>[2x]MKPHNSEKYFVKNGQPHFLISGEVHYFRINPKLWRNHLQLLKQTGADTVSTYIPWDWHEIEEDDFDFEGKTHPARNLIRFIKLCKEENLDLIVKPGPYILAEYENQGLPSWLLKKLSKNAFALDENGNVISPDLVSYLSDEFLEYTFKWYDKVMPIISKHQKEHYGPITMMQLCNEIGVFQWLSGKSDYNPKVINLYKEFIIQRYKTIEKLNSVYSTNYNSFDDLKAPSGKIKLRSDYCAYFDFHLFFREYYNKYISILKNKIRSFGINIKLTHNIPGWIYGNASELPMLISTYSEIMKNHPDIIFGLDHIPEFVSFRNAHSDLACNKILEAMQPEAPVWAAQFQAGTREHHVKAYAKDLETFYIASLAHGIKGFNYYMFSQGINPEGKGFYGKTFYFQTALDAASNKLALYDSIKKVNRFIRKEQKDLLRTNVNSEICVGFYKPYFFTELISSQLLKEKKLNVEELGLYIDPRFLREEILFNGLLRGLQTLNYNYDVVDLENCDLKSLTAYKQLWITSAEFMDAETQNLLSEFVLNGGNLILYPAVPTLDNYLNRCEILKNNFGIEFITKDSSHKVSAFGIEDVFTAFSKKQIYNDTNSKPIAFTQENEICGIRKKIGKGELTILGFAFGYTSDEHLELIDKLVKLNKIKRELFVSDKDIQFVVRENNKSRYIFFLNYHNERKTFNYRKSSELKKKKSEEISIAPFSYKVIKENKLEHHHHHH

The IALB_1185 protein, which is encoded in the gene cluster for endo-β-1,2-glucanase homologs in the genome of Ignavibacterium album, is a glycoside hydrolase family (GH) 35 protein. Here, we showed using recombinant IALB_1185 that this protein has glycosyltransferase activity toward β-1,2-glucooligosaccharides, and that the kinetic parameters for β-1,2-glucooligosaccharides are not within the ranges for general GH enzymes. Kinetic analysis further revealed that the enzyme has wide aglycone specificity regardless of the anomer, and that the β-1,2-linked glucose dimer sophorose is an appropriate donor. We propose that IALB_1185 be redefined β-1,2-glucooligosaccharide:d-glucoside β-d-glucosyltransferase as a systematic name and β-1,2-glucosyltransferase as an accepted name.

Thus, crystals of the E343Q mutant (the mutant of the nucleophile) were soaked in a solution containing Sop4. Clear electron density fitting a Sop2 molecule was observed at subsites +1 and +2 only in subunit A. An electron density beyond subsite +2 is almost absent in the solvent, suggesting that there is no subsite +3 in IaSGT. Importantly, as shown later, electron density fitting ligands was not observed at subsite −1 at all. The Glc moiety at subsite +2 is hydrogen-bonded with the side chain of Gln106 and the main chain of Glu102. The aromatic ring of Phe391 undergoes hydrophobic interaction with the C6 atom in the moiety. In the WT-Sop2 complex, both the side chain carboxy group oxygen atoms of Glu102 participate in the substrate recognition at subsite −1. However, the distance between one of the oxygen atoms in Glu102 and a potential hydrogen atom generated from the C3 atom of the Glc moiety at subsite +2 by PyMOL (2.2 Å) is outer limit for van der Waals distance between nonbonded hydrogen and oxygen atoms. The distance is smaller than the normally allowed one (2.4 Å), as shown as overlapped spheres. This observation suggests that binding at subsites −1 and +2 competes mildly through Glu102.> STSDRLKAVEQNLYDVGPRDSGGREGPGHYIAISGNTAAGKTTLIETLAGSLRAAGADAVGVSERVFHHRYLKLMFSASADFAFPIQLSFMLERHLLLLDNLVRRGRTMVMERSHLDDAMFVREHVASGAIT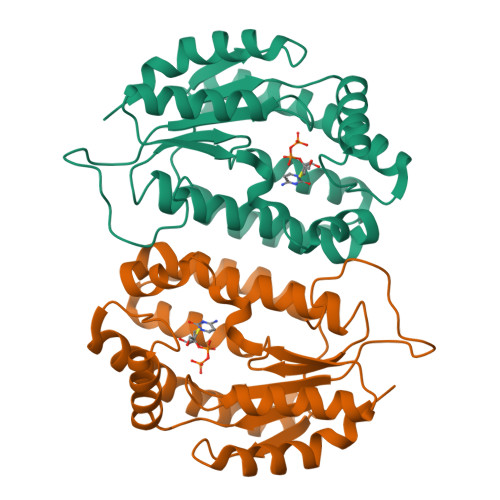AAQQRAYTEVSGELNARIPNPDLIVLMNPEPELSLERLARAEAEGSRPRQFPSDAAKRAWVHRWYDLYQELHDDYRRRAVDGDLRGTELLELDAAASPEEKIATVTARARSLVVG> ARVTVQDAV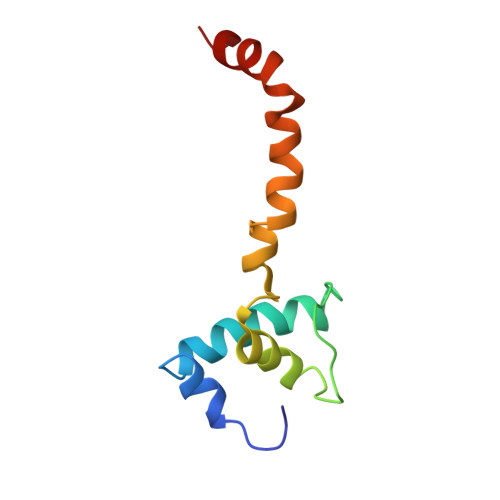EKIGNRFDLVLVAARRARQMQVGGKDPLVPEENDKTTVIALREIEEGLINNQILDVRERQEQQEQEAAELQAVTAIAEGRR> MHHHHHHGENLYFQGSLRIAKEALTFDDVLLVPAHSTVLPNTADLSTQLTKTIRLNIPMLSAAMDTVTEARLAIALAQEGGIGFIHKNMSIERQAEEVRRVKKHSGGLRVGAAVGAGAGNEERVDALVAAGVDVLLIDSSHGHSEGVLQRIRETRAKYPDLQIIGGNVATAAG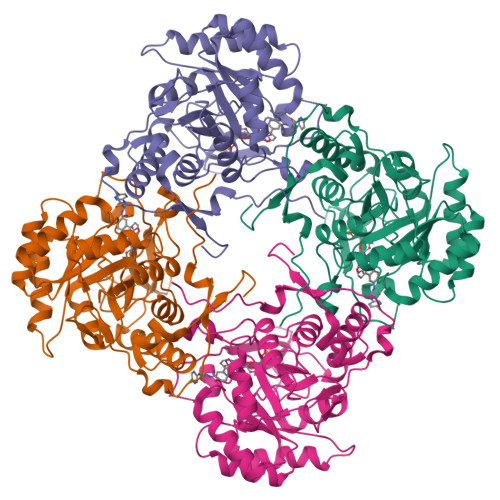ARALAEAGCSAVKVGIGPGSICTTRIVTGVGVPQITAVADAVEALEGTGIPVIADGGIRFSGDIAKAIAAGASAVMVGSMLAGTEESPGEIELYQGRSYKSYRGMGSLGAMSKGSSDRYFQSDNAADKLVPEGIEGRVAYKGRLKEIIHQQMGGLRSCMGLTGCGTIDELRTKAEFVRISGAGIQESHVHDVTITKESPNYRLGSGNS> MKAKKTLNMITQRAVEEGIAMEIGKTSRQYFDACSIIEMNEQDMKELGIMKNTNVRVK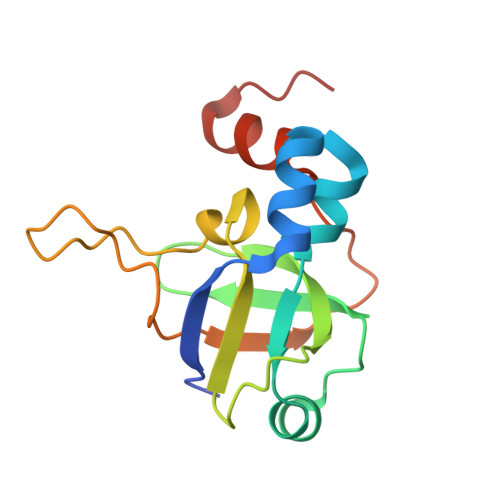SESGEVVVKAVVGRQTCYPGLCHIRQGVWANQVVPPRTQSTGAPQYSGFPVTVEPVPNERLKTALELVQGAVGMWKGDQ> MEDISEPPLHDFYCSRLLDLVFLLDGSSRLSEAEFEVLKAFVVDMMERLRISQKWVRVAVVEYHDGSHAYIGLKDRKRPSELRRIASQVKYAGSQVASTSEVLKYTLFQ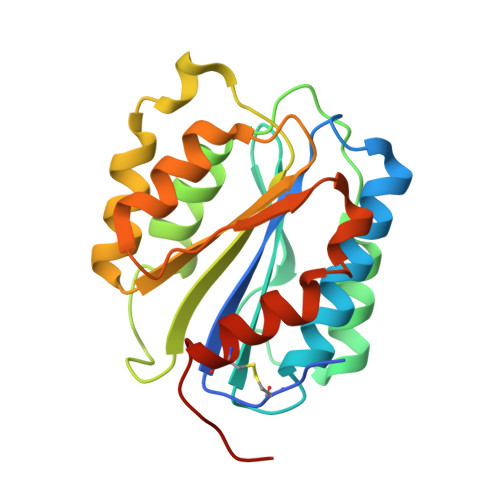IFSKIDRPEASRIALLLMASQEPQRMSRNFVRYVQGLKKKKVIVIPVGIGPHANLKQIRLIEKQAPENKAFVLSSVDELEQQRDEIVSYLCDLAPEAPPPTLPPH>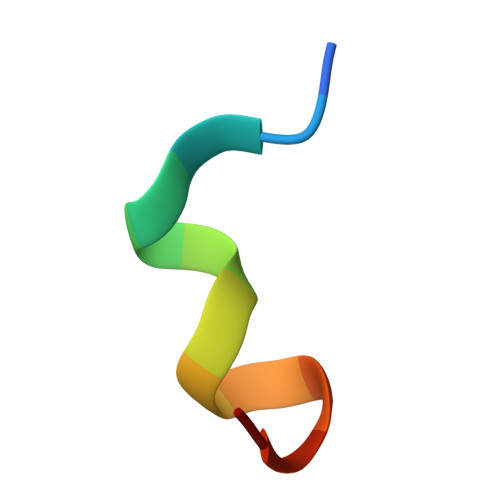 AFPDYLAEYHGGX(1'S)-2',3'-dihydrospiro[imidazolidine-4,1'-indene]-2,5-dione | C11 H10 N2 O2 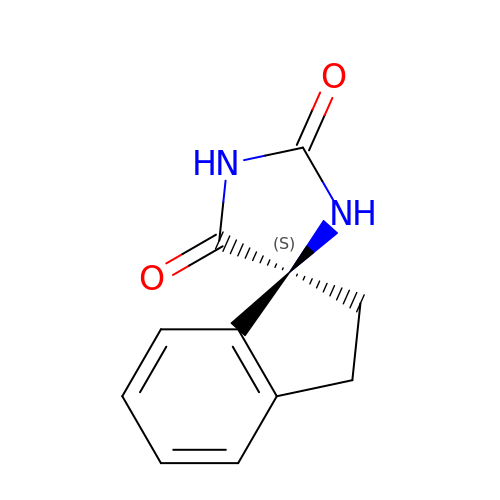| CDALGRHRPPTQPM-NSHDSACASA-N>MHHHHHHMNPDLRRERDSASFNPELLTHILDGSPEKTRRRREIENMILNDPDFQHEDLNFLTRSQRYEVAVRKSAIMVKKMREFGIADPDEIMWFKNFVHRGRPEPLDLHLGMFLPTLLHQATAEQQERFFMPAWNLEIIGTYAQTEMGHGTHLRGLETTATYDPETQEFILNSPTVTSIKWWPGGLGKTSNHAIVLAQLITKGKCYGLHAFIVPIREIGTHKPLPGITVGDIGPKFGYDEIDNGYLKMDNHRIPRENMLMKYAQVKPDGTYVKPLSNKLTYGTMVFVRSFLVGEAARALSKACTIAIRYSAVRHQSEIKPGEPEPQILDFQTQQYKLFPLLATAYAFQFVGAYMKETYHRINEGIGQGDLSELPELHALTAGLKAFTSWTANTGIEACRMACGGHGYSHCSGLPNIYVNFTPSCTFEGENTVMMLQTARFLMKSYDQVHSGKLVCGMVSYLNDLPSQRIQPQQVAVWPTMVDINSPESLTEAYKLRAARLVEIAAKNLQKEVIHRKSKEVAWNLTSVDLVRASEAHCHYVVVKLFSEKLLKIQDKAIQAVLRSLCLLYSL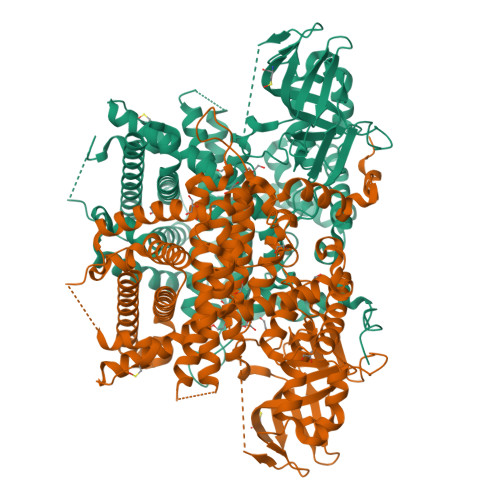YGISQNAGDFLQGSIMTEPQITQVNQRVKELLTLIRSDAVALVDAFDFQDVTLGSVLGRYDGNVYENLFEWAKNSPLNKAEVHESYKHLKSLQSKL[2x]> MMRKSVTFLRRGKPRPRAGMFPDKYRRVPMLLKPQQGGQQYFNHFLIRSTNDRLTQQDVD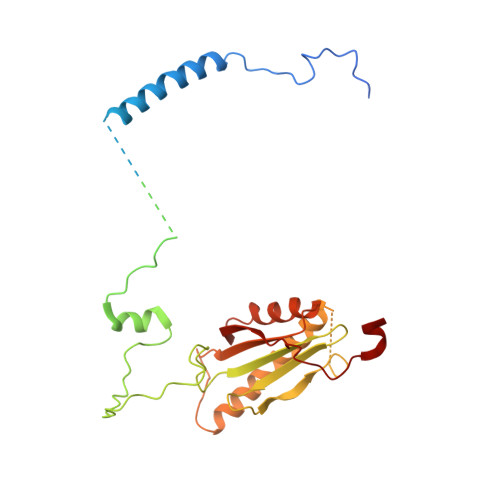NASGQAHSFISPQLPQMDWRNMSARSSEESIREEMRQLAENDVMQHQRVFNERMWYEKEEEHRMKARSCPEETSEHAISNDGAVPPPRVLGGDYFKTRFGYSLVKNSEMTQGPVDYSQLDMWGEMPRYTSDMVFLYLVSRRRNTYAVAYTYEGKRILNTYTAGNRGLKGGDRGFRSEGSTDNGHQVTSMYLNDLLPKLREMRASEGRPMGRGEKVELVVRVMGFYNGRQGAVRAVQDRANEFHVRYFEDITPFPLNGPKMPRGVFK>[2x]GQYKDNIRHGVCWIYYPDGGSLVGEVNEDGEMTGEKIAYVYPDERTALYGKFIDGEMIEGKLATLMSTEEGRPHFELMPGNSVYHFDKSTSSCISTNALLPDPYESERVYVAESLISSAGEGLFSKVAVGPNTVMSFYNGVRITHQEVDSRDWALNGNTLSLDEETVIDVPEPYNHVSKYCASLG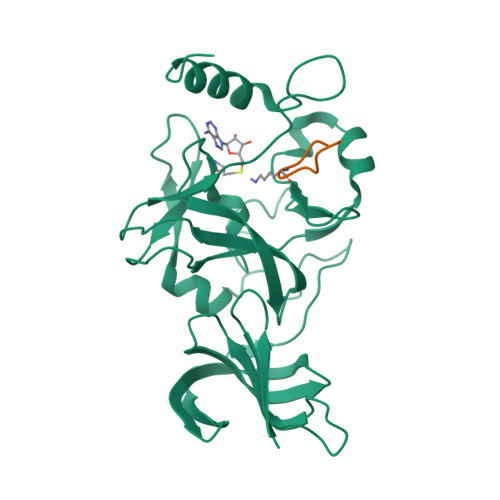HKANHSFTPNCIYDMFVHPRFGPIKCIRTLRAVEADEELTVAYGYDHSPPGKSGPEAPEWYQVELKAFQATQQK;>[2x]ARTKQTARKY Like other Paramyxoviridae, RSV has a non-segmented negative sense RNA genome that is coated by the viral nucleoprotein N to form the nucleocapsid (NC), which serves as the template for RNA synthesis by the viral RNA-dependent RNA polymerase. The structure showed that the N-protein has a core region composed of N- and C-terminal domains (the ‘N-core’), with the RNA bound in a groove between them. In addition, an N-terminal and a C-terminal extension, called N-arm (residues 1–28) and C-arm (residues 360–375), invade the 5′ and the 3′ adjacent subunits in the RNA-bound ring, respectively. The NC is a flexible helix, with variable pitches and numbers of N-proteins per turn of the helix.

Here we set out to determine unequivocally the handedness of the helical RSV NC by electron tomography of purified NC-like ribonucleoprotein complexes (RNPs). The resulting reconstructions showed that both MeV and RSV NC-like helical RNPs are left-handed, with a pitch of 52 Å and 68 Å, respectively. A composite subunit was assembled including the coordinates of the N-core and seven RNA nucleotides most closely bound to it, together with the N- and C-arms of its immediate neighbours on either side. Although the close contacts of the N-core with its neighbours are scarce, there are a few key contacts between N-core atoms, in particular the interactions of the Arg234 side-chain, which links three consecutive subunits. Thus, Arg 234 from subunit N−1 makes a bidentate salt bridge with the Asp221 side-chain of N0 whilst simultaneously hydrogen bonding the side-chain of Tyr23 in the N-arm of the second neighbour along the chain (N+1) (the subunits are numbered in the 5′ to 3′ direction of the RNA along the ring). Modelling the helix using the COM of the Cα of Asp221 and Tyr23 from protomers on each side of the subunit as the centre of rotation about the radial axis, rather than rotating about the COM of the whole subunit, resulted in a model for the helical NC with minimal clashes that preserved the inter-subunit hydrogen bonding described above. Superposing the N-core of one subunit in the ring with its counterpart in the final helical NC resulted in a root mean square deviation (r.m.s.d.) of 3.9 Å between Cα atoms in the immediate corresponding neighbour, with the largest displacement of about 8 Å. We have demonstrated that RSV has a left-handed NC, a feature that is in common with other Mononegavirales. The most important implication of this finding is that the 3′ end of the RSV genome is located at the pointed end of the NC, and not at the barbed end.

>[23x]MALSKVKLNDTLNKDQLLSSSKYTIQRSTGDSIDTPNYDVQKHINKLCGMLLITEDANHKFTGLIGMLYAMSRLGREDTIKILRDAGYHVKANGVDVTTHRQDINGKEMKFEVLTLASLTTEIQINIEIESRKSYKKMLKEMGEVAPEYRHDSPDCGMIILCIAALVITKLAAGDRSGLTAVIRRANNVLKNEMKRYKGLLPKDIANSFYEVFEKHPHFIDVFVHFGIAQSSTRGGSRVEGIFAGLFMNAYGAGQVMLRWGVLAKSVKNIMLGHASVQAEMEQVVEVYEYAQKLGGEAGFYHILNNPKASLLSLTQFPHFSSVVLGNAAGLGIMGEYRGTPRNQDLYDAAKAYAEQLKENGVINYSVLDLTAEELEAIKHQLNPKDNDVEL6-ethyl-3-[[3-methoxy-4-[4-(4-methylpiperazin-1-yl)piperidin-1-yl]phenyl]amino]-5-(oxan-4-ylamino)pyrazine-2-carboxamide | C29 H44 N8 O3 | 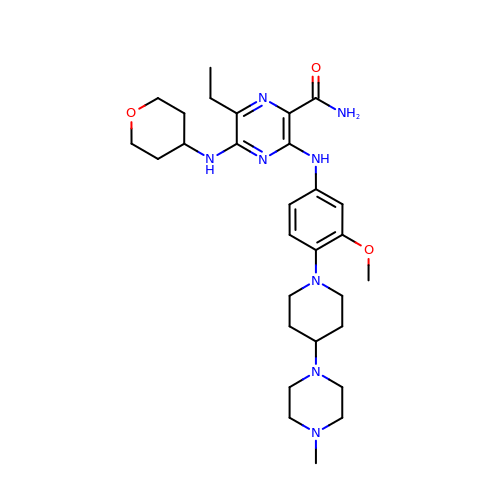GYQYAJJFPNQOOW-UHFFFAOYSA-N> MRGSAVPPTYADLGKSARDVFTKGYGFGLIKLDLKTKSENGLEFTSSGSANTETTKVTGSLETKYRWTEYGLTFTEKWNTDNTLGTEITVEDQLARGLKLTFDS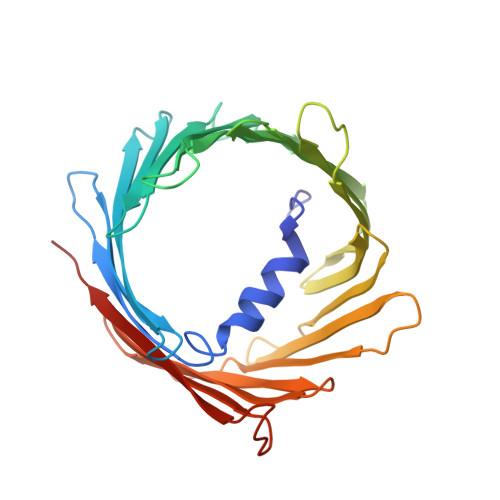SFSPNTGKKNAKIKTGYKREHINLGCDMDFDIAGPSIRGALVLGYEGWLAGYQMNFETAKSRVTQSNFAVGYKTDEFQLHTNVNDGTEFGGSIYQKVNKKLETAVNLAWTAGNSNTRFGIAAKYQIDPDACFSAKVNNSSLIGLGYTQTLKPGIKLTLSALLDGKNVNAGGHKLGLGLEFQARSHHHHHH>[12x]PIMGQDVKYLFQSIDAATGSAPLFPA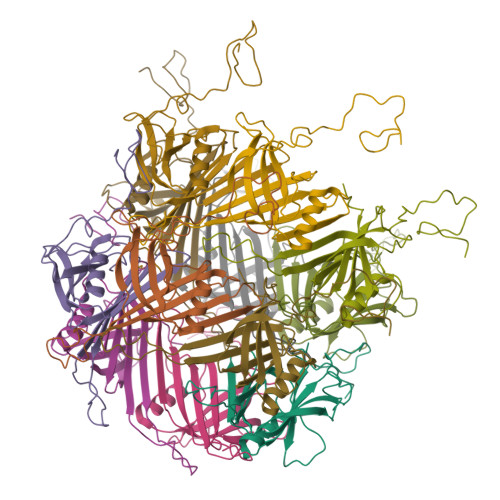YQTDGSVSGERELFDEQTKNGRILGPGSVADSGEVTYYGKRGDAGQKAIEDAYQNGKQIKFWRVDTVKNENDKYDAQFGFAYIESREYSDGVEGAVEISISLQVIGELKNGEIDTLPEEIVNVSKGGYDFQQPGQTTGEAPGTVPA> MAKRVADAQIQ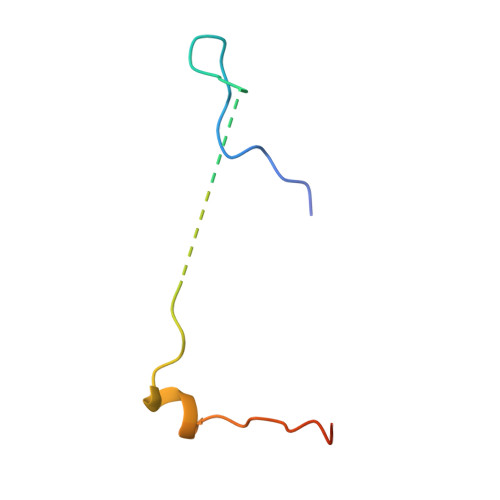RETYDSNESDDDVTPSTKVASSAVMNRRKIAMPKRRMAFK>MGHHHHHHMPMYEVQWKVVEESNGNNYSYIDPTQLPYDHKWEFPRNRLSFGKTLGAGAFGKVVEATAQGLIKSDAAMTVAVKMLKPSAHSTEREALMSELKVLSYLGNHENIVNLLGACTHGGPTLVITEYCCYGDLL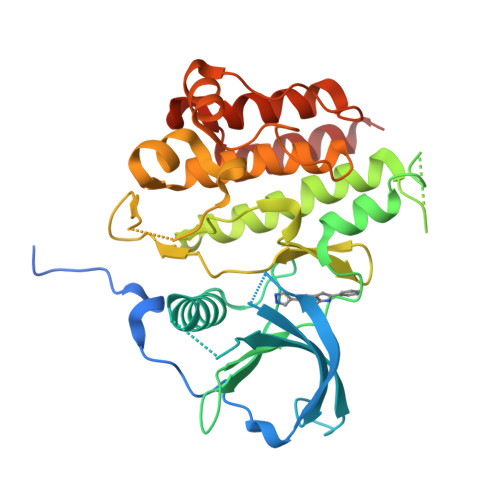NFLRRKRDSFHSSDTSPASMEDDENALDLEDLLSFSYQVAKGMAFLASKNCIHRDLAARNILLTHGRITKICDFGLARVIKNDSNYVDKGNARLPVKWMAPESIFNSVYTFESDVWSYGIFLWELFSLGSSPYPGMPVDSKFYKMIKEGFRMSSPEHAPAEMYDIMKTCWDADPDKRPTFKQIVQDIEKQISESTNH[2x]DEQUALINIUM | 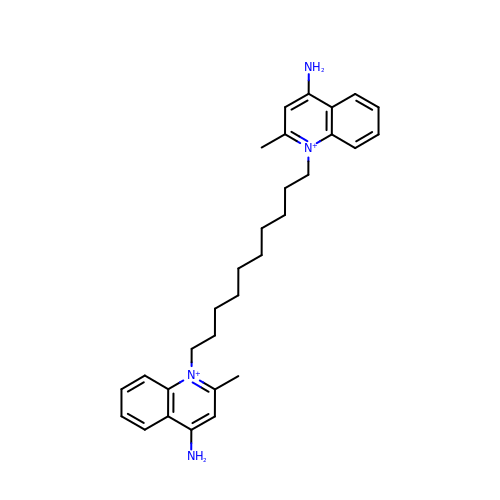C30 H40 N4 | PCSWXVJAIHCTMO-UHFFFAOYSA-P>[2x]AALENPGTVEELHKKCKDIQAITFEGAKIMLNKGLSNHFQVSHTINMSNVVPSGYRFGATYVGTKEFSPTEAFPVLLGDIDPAGNLNANVIHQFSARLRCKFASQIQESKVVASQLTTDYRGSDYTLSLTVANPSIFT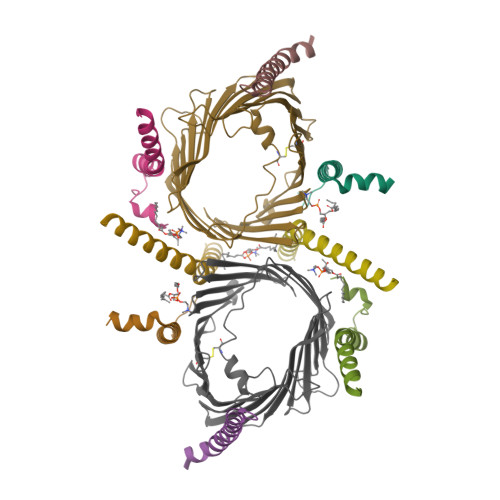NSGVVVGQYLQSVTPALALGSELAYQFGPNVPGRQIAIMSVVGRYTAGSSVWSGTLGQSGLHVCYYQKASDQLQIGAEVETSLRMQESVATLAYQIDLPKANLVFRGGIDSNWQIFGVLEKRLAPLPFTLALSGRMNHVKNNFRLGCGLMIG;>[2x]ATVKSVKGFYSFSCNASWIFFTSAVILFAPVIFETERAQMEELHKSQ;>[2x]DRLGFVVGVVQTGFHWGFVPLVLYLGFMKGAEPGMPPLNLFSLLWQ;>[2x]PLSIVRSIYNNEFQWMLVKSYGLFFLGVRLAKEFVGVELMPS;>SQPDPAEEQKRVAAEVRFNFILFGAVIAAVRLAPIVLKH[2x]> MDDFNNILDLLINESKKAAQLGDIPVSCCIIDSNNNILSLAINSRYKNKDISQHAEINVINDLISKLNSFNLSKYKLITTLEPCMMCYSAIKQVKINTIYYLVDDPKKNNYSINDQNLNLIQIKNQKKQSEYIKLLNIFFINARLEHHHHH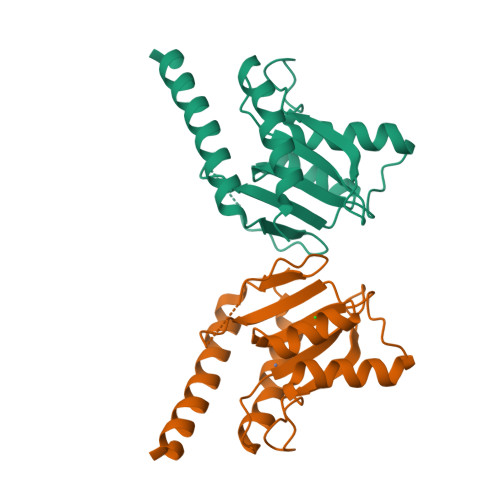H> MRYLKIEKEKLVSCKKQEQEVQRIRRRKGNQKLNSIAKQQRVKRRDYQQNIKQNKEVKNPKKLIKQQIINKVKKRKKMFRGLTKFNKVFALNSFKNSLVAVPKANLNHVQNMLEENLKYDAQKYNDEVAVIQKTSRIYKPTYTIEFNREGEVLVYSADPIKNSVVYFKYPYVLYEAAIPLFIWAWIYNPLELSKNAVNSLLIYPNIAWI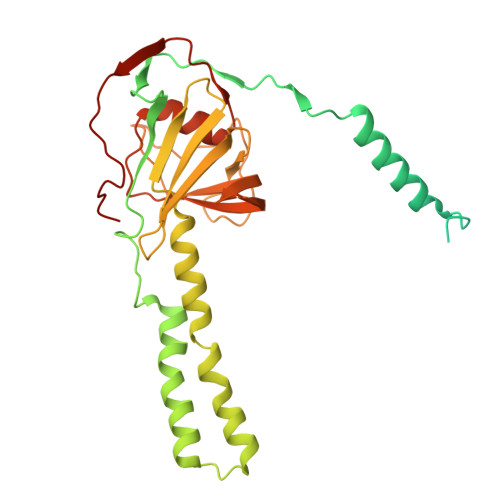PRMWYWRSLQYKIQKMYLLRGGKVAKIETQSLAGDRFTSWVETYQFHPLTQDQKNFDNQDNAEFLEDEGQLKYELGVQLDNLQEMGTTSQDIVINFMKEGTVHHPELFEAIVKGYNIDTSDYVINTANNLRAREGNHNH> GHMAKTYDYLFKLLLIGDSGVGKTCVLFRFSEDAFNSTFISTIGIDFKIRTIELDGKRIKLQIWDTAGQERFRTITTAYYRGAMGIMLVYDITNEKSFDNIRNWIRNIEEHASADVEKMILGNKCDVNDKRQVSKERGEKLALDYGIKFMETSAKANINVENAFFTLARDIKAKMDKKLEGNSPQGSNQGVKITPDQQKRSSFFRCVLL;> GHMKQEELKRLYKAQAIQRQLEEVEERQ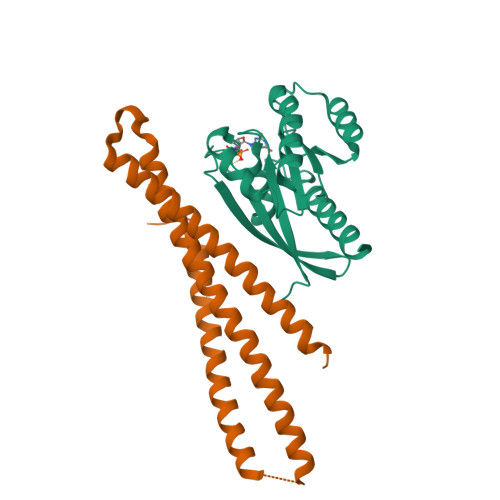RASEIQGVRLEKALRGEADSGTQDEAQLLQEWFKLVLEKNKLMRYESELLIMAQELELEDHQSRLEQKLREKMLKEESQKDEKDLNEEQEVFTELMQVIEQRDKLVDSLEEQRIREKAEDQHFES> MTTLTRQDLNFGQVVADVLSEFLEVAVHLILYVREVYPVGIFQKRKKYNVPVQMSCHPELNQYIQDTLHCVKPLLEKNDVEKVVVVILDKEHRPVEKFVFEITQPPLLSINSD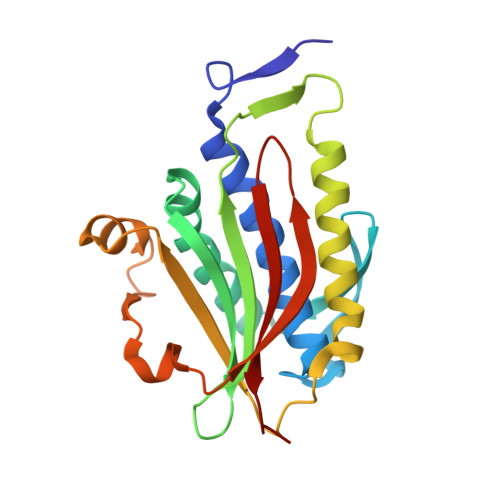SLLSHVEQLLAAFILKISVCDAVLDHNPPGCTFTVLVHTREAATRNMEKIQVIKDFPWILADEQDVHMHDPRLIPLKTMTSDILKMQLYVEERAHKN>[2x]SMKHPLEELKDPTENLLLWIGRFLRYKCTSLSNSQVKDQNKVFECLNELNQACSSSQLEKVCKKARNAGLLGINTYALPLLKFHEYFSKARLITERLAFNSLKNIDEVMLAEFLSVYTGGLSLATKKNYRIALLGLFSYIDKQNQDENEKSYIYNITLKNISGVNQSAGNKLPTHLNNEELEKFLESIDKIEMSAKVRARNRLLIKIIVFTGMRSNEALQLKIKDFTLENGCYTILIKGKGDKYRAVMLKAFHIESLLKEWLIERELYPVKNDLLFCNQKGSALTQAYLYKQVERIINFAGLRREKNGAHMLRHSFATLLYQKRHDLILVQEALGHASLNTSRIYTHFDKQRLEEAASIWEEN

In bacteria and archaea, chromosome dimers are monomerized by members of a large family of tyrosine recombinases, the Xer recombinases. Many other organisms (including Lactococcus, Helicobacter, Campylobacter spp. and archaea) employ a single Xer recombinase system, with a prime example, XerH/difH, found in Helicobacter pylori, a gastric pathogen implicated in peptic ulcer disease and gastric cancer. Xer recombinases are members of the tyrosine site-specific recombinase superfamily, a large group of enzymes that catalyze DNA breakage and rejoining using a conserved tyrosine nucleophile. Here, we present two crystal structures of the H. pylori XerH recombinase in complex with its recombination site difH.

Attempts to co-crystallize XerH with suicide versions of the native difH sequence were unsuccessful, but palindromic difHLP suicide substrates gave us crystals that diffracted to 2.4 Å. Most strikingly, the difH DNA is now strongly bent. The bend mainly originates from a single distortion within the central region of difH: bases A17’ and G18’ are un-stacked with a 90° tilt, which introduces a kink resulting in asymmetric bending of the DNA (insert in Figure 4B). Each subunit is rotated by ~22° in the post-cleavage structure, resulting in major rewiring of the inter-subunit interactions and an overall compaction of the complex. At the same time, helices αN and αO of molecule A are rotated by ~30°, bringing the catalytic Y344 to a suitable position to attack one strand on each difHLP DNA forming a covalent phosphotyrosyl bond (left). Interestingly, despite the symmetry of the palindromic difHLP substrate, the two bound XerH molecules (A and B) are in different conformations. Their overall structures are similar (r.m.s. deviation 0.78 Å for Cα carbons), but important protein segments that contain catalytic residues (the β2-β3 turn with K239, and αN-αO carrying Y344) are in different conformations. Consequently, subunit A assumes a fully active conformation, while subunit B is in an inactive conformation with the catalytic tyrosine distant from the scissile phosphate. In the active subunit (molecule A, left), R213, H309, R312, and H335 make hydrogen bonds with the scissile phosphate (orange), K239 contacts the base of the adjacent nucleotide A12, and Y344 is covalently attached to the DNA.PENTANE-3,4-DIOL-5-PHOSPHATE | C5 H13 O6 P | 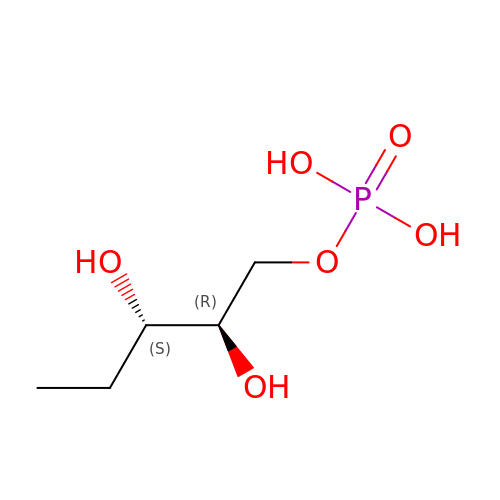FQKLTSRHTQGSQZ-CRCLSJGQSA-N> MGKKTFREWQYFKLSITSFDQDVDDAHAIDQMTWRQWLNNALKRSYGIFGEGVEYSFLHVDDKLAYIRVNHADKDTFSS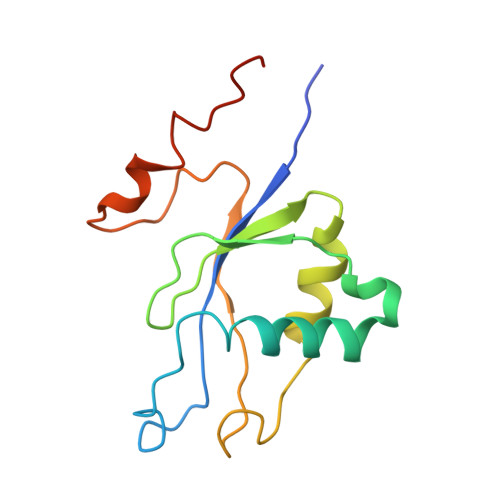SISTYISTDELVGSPLTVSILQESSSLRLLEVTDDDRLWLKKVMEEEEQDCKCI>[2x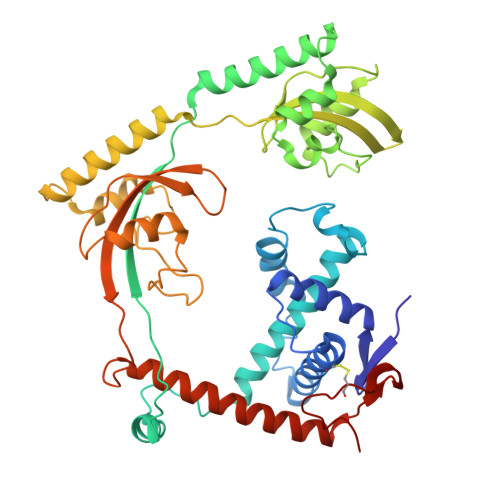]IDEVVWVIGDEAILKSDVEEARLAALYEGRKFDGDPYCVIPEELAVQKLYMHQAVLDSIEVPEAEVIQRVDYQINNYIQAMGTREKLEEYFNKTSTQIREAMRENARDGLIVQRMQQKLVGDIKVTPAEVRRYFKELPQDSIPYVPTQVEVQIITQQPKIPVAEIEDVKRRLREYTDRINKGESDFSTLALLYSEDRGSAIKGGETGFMGKGQMVPEYANVAFNLQDTKKISKIVESEYGFHIIQLIEKRGDRINTRHILLKPKVSDKELDEANARLDSIANDIRSDKFTFDQAASALSQDKDTRNNHGLMQNPQNQTAKFEMQDLPQEIAKVVDKMNIGEISKAFTMVNPKDGKEVCAIVKLKSRINGHKATITDDYQNLKEIVLDKRREEALQKWIVEKQKHTYVRINPAWQRCDFKYPGWIKKD>MHHHHHHRFDIPGYELVYTAPVETALQADDLRNTAEVWQQMFDAAKTRIDLGQFYVANQQGSLLDGVLQHLKAAGERGVKIRFLMEEKGIRLSTPETLEQLKAIPNLELRIIPYRRLSGGILHAKYLLVDGEQAFVGSQNFDWRALEHIHETGLRISDAGV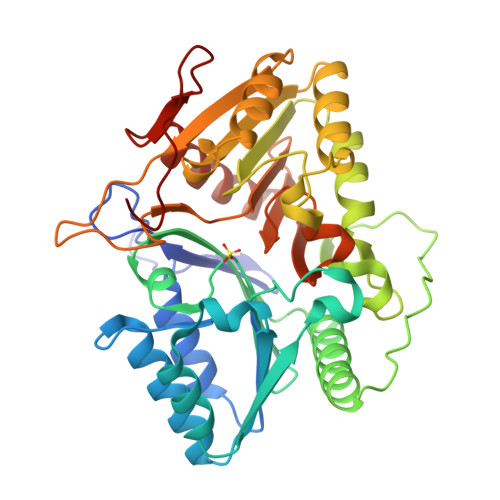VGQIQAIFEQDWRAQALLTADKPVPQLTYQPTAATPQGNYLVASPRAYNPAGVIDSQVELPRLLASAKQRVRVQVMDYAPLSYGPERSRPYYAVIDNALRSAAARGVQIELMVANWNTKKPDIAWLKSLALVPNVQIKVVTIPPASHGFIPFARVIHSKLMTIDGETAWVGTSNWTGGYLDNSRNLELVLHSPAMSQRLDTLYSQLWDSVYAEPIKLDYDYPAPKPGGES[2x]> SPTVEACGYSDRIIQITRGDSTITSQDVANAIVAYGVWPHYLSSKDASAIDKPSQPDTSSNRFYTLRSVTWSSSSKGWWWKLP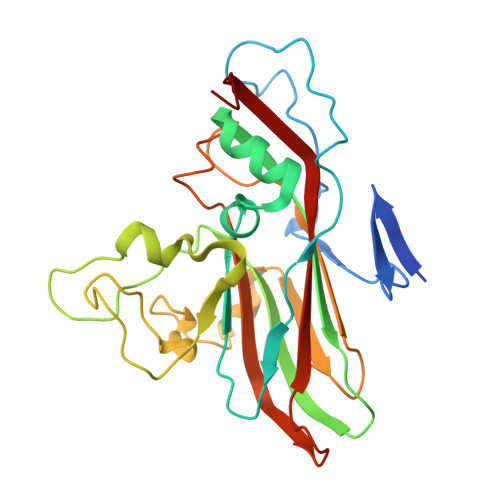DALKDMGIFGENMFYHYLGRSGYTIHVQCNASKFHQGTLIVALIPEHQIASALHGNVNVGYNYTHPGETGREVKAETRLNPDLQPTEEYWLNFDGTLLGNITIFPHQFINLRSNNSATIIAPYVNAVPMDSMRSHNNWSLVIIPICPLETSSAINTIPITISISPMCAEFSGARAKRQ> GPHNMATLTDRTYLPPLEDCLTGRTVILSWRLVASALEDADLARLTSPALSTFLRDGFVHELLKHPARVFEPKDLKQEFETKTSSIQTVAPGVDTIKKDALWLADAVAINQVAALRIVLIEYQTRAHSHLVLPLSTQDVANIQEAAGVGDAHASSILSLLNPASAVDAETMWCDFETEARRRERILATYLSERRSFTAAVDALVTFLLHSAPGQHKDLDSLRRALLKDAFAFDEDLDVPDRSKLLTMAPTYMNLVEDCIARA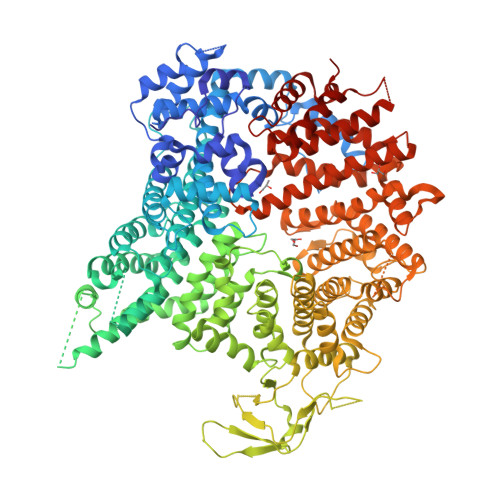QALPAKLGESFKTEAFELDWLRTAITEAVHSLSIAFQALDLDTPYFAPHELLSEWFELMNSSLFLESILGFEVVADLAMPARSLVSAICLKMLNIDRTIQFLHDFDYPDGEEPYLLSSQTLNKIHTAVTNAVNSGVAASLPVAFAWSLIVHQMHLGYQERAERRDLLVNQRAQAGFELEFQPSASTPNRRRRNSAGSIVSLEASPYDDFLREQRLDNDIAPVEQIAMLATSRGQVYQVMSEMALCLGTTHEAAFRPAVGARARLVFQDLLKRSAYLIPYQDEPVFSLLAILATGRQYWDVTDALSASSLNQVYTDMLDDETLFTQFTMQAINRFPYEFNPFSVLCRVLAAALITNKDKADVVTGWLWRTPTLTVDWNPAWDRSYELCFEDENTNSFRLTRDVDLFGSASPARPRHLAAEERFIIPEGTLGRFVTDVGRTARLEFEHSALALLGKRLEVKAAEEICDSGMAPLDVDEQAEAVAMLATVLRAESLKSTAKGGDPEAPLKFLKEASRLLPHNKDILTVISDTIDGLVEKELLELDGPQIAVLASCLQFLHAALAVCPGRVWAYMSRCALIAGDARPGRLSRITGSLDMYAERFDLLSSAVKLFAALIDSAACSAVQRRAGSTALVSVRSAVENPWLGTSEKILSRVALAIAQAALDVYESTTTWRFRSELDRSILVRDVVGLMHKLVVHAHTLSSHLTSTLSPAAAHIISSFLTPPPSASSLRFQPLLGTLLVALITPRATLYPGQSRILAERVTSVLAFCTSLLRAADFLGQTHIPLQTHLFQSACLLARLPAANAVYRAPVLELLRALVEVAGRAANGSGEPPSLLGYLGSHAARSFISLVEGIDKPFGRVEHAVVTWRFFAAVIRN The CST–Polα/primase complex is essential for telomere maintenance and functions to counteract resection at double-strand breaks. In addition to its telomeric function, CST–Polα/primase performs an analogous fill-in reaction at resected double-strand breaks (DSBs). We report a 4.6-Å resolution cryo-EM structure of human CST–Polα/primase, captured prior to catalysis in a recruitment state stabilized by chemical cross-linking. Our structure reveals an evolutionarily conserved interaction between the C-terminal domain of the catalytic POLA1 subunit and an N-terminal expansion in metazoan CTC1.

We purified Polα/primase lacking POLA1N (referred to hereafter as PPΔN), reconstituted a CST–PPΔN(–ssDNA) complex as for full-length Polα/primase (referred to hereafter as PPFL), and collected cryo-EM data. We used 131,850 particles to generate the final map with a global resolution of 4.6 Å. The ssDNA was included in the complex, as evidenced by the native gel of the GraFix fractions, but no reliable density could be found for it owing to the low resolution of CST in the cryo-EM map. After initial rigid-body docking followed by flexible fitting and refinement, the overall conformations of the two subcomplexes did not show major changes from their structures in isolation. Thus, we conclude that our structure likely captures a recruitment state of the complex that forms prior to active RNA and DNA synthesis by Polα/primase. The primary interaction interface observed in our structure occurs between the C-terminal domain of POLA1 (POLA1CTD, 1,265–1,462 aa) and the N-terminal OB folds of CTC1. The resolution is limiting for rigorous analysis of amino acid interactions, and analysis of surface electrostatic potential suggests that this interface is not driven by a dominant hydrophobic or charged interaction, but rather by shape complementarity of the two proteins, burying 1,250 Å2 of solvent-accessible surface area. The CRL and one Zn2+-binding domain in POLA1CTD form the module that fits into a complementary cleft in CTC1. CTC1OB-D, an elongated OB fold that shares no homology with known OB folds, forms the major interaction with POLA1CTD. V665 resides on a β-strand of CTC1OB-D, so it is plausible that a glycine substitution would destabilize the β-sheet and OB fold, disrupting the primary interaction.

> METFDPTELPELLKLYYRRLFPYSQYYRWLNYGGVIKNYFQHREFSFTLKDDIYIRYQSFNNQSDLEKEMQKMNPYKIDIGAVYSHRPNQHNTVKLGAFQAQEKELVFDIDMTDYDDVRRCCSSADICPKCWTLMTMAIRIIDRALKEDFGFKHRLWVYSGRRGVHCWVCDESVRKLSSAVRSGIVEYLSLVKGGQDVKKKVHLSEKIHPFIRKSINIIKKYFEEYALVNQDILENKESWDKILALVPETIHDELQQSFQKSHNSLQRWEHLKKVASRYQNNIKNDKYGPWLEWEIMLQYCFPRLDINVSKGINHLLKSPFSVHPKTGRISVPIDLQKVDQFDPFTVPTISFICRELDAISTNEEEKEENEAESDVKHRTRDYKKTSLAPYVKVFEHFLENLDKSRKGELLKKSDLQKDF;> GGSMEFSGRKWRKLRLAGDQRNASYPHCLQFYLQPPSENISLIEFENLAIDRVKLLKSVENLGVSYVKGTEQYQSKLESELRKLKFSYRENLEDEYEPRRRDHISHFILRLAYCQSEELRRWFIQQEMDLLRFRFSILPKDKIQDFLKDSQLQFEAISDEEKTLREQEIVASSPSLSGLKLGFESIYKIPFADALDLFRGRKVYLEDGFAYVPLKDIVAIILNEFRAKLSKALALTARSLPAVQSDERLQPLLNHLSHSYTGQDYSTQGNVGKISLDQIDLLSTKSFPPCMRQLHKALRENHHLRHGGRMQYGLFLKGIGLTLEQALQFWKQEFIKGKMDPDKFDKGYSYNIRHSFGKEGKRTDYTPFSCLKIILSNPPSQGDYHGCPFRHSDPELLKQKLQSYKISPGGISQILDLVKGTHYQVACQKYFEMIHNVDDCGFSLNHPNQFFCESQRILNGGKDIKKEPIQPETPQPKPSVQKTKDASSALASLNSSLEMDMEGLEDYFSEDS;> GPGSADEEQVFHFYWLDAYEDQYNQPGVVFLFGKVWIESAETHVSCCVMVKNIERTLYFLPREMKIDLNTGKETGTPISMKDVYEEFDEKIATKYKIMKFKSKPVEKNYAFEIPDVPEKSEYLEVKYSAEMPQLPQDLKGETFSHVFGTNTSSLELFLMNRKIKGPCWLEVKSPQLLNQPVSWCKVEAMALKPDLVNVIKDVSPPPLVVMAFSMKTMQNAKNHQNEIIAMAALVHHSFALDKAAPKPPFQSHFCVVSKPKDCIFPYAFKEVIEKKNVKVEVAATERTLLGFFLAKVHKIDPDIIVGHNIYGFELEVLLQRINVCKAPHWSKIGRLKRSNMPKLGGRSGFGERNATCGRMICDVEISAKELIRCKSYHLSELVQQILKTERVVIPMENIQNMYSESSQLLYLLEHTWKDAKFILQIMCELNVLPLALQITNIAGNIMSRTLMGGRSERNEFLLLHAFYENNYIVPDKQIFRKPQQKLGDEDEEIDGDTNKYKKGRKKAAYAGGLVLDPKVGFYDKFILLLDFNSLYPSIIQEFNICFTTVQRVASEAQKVTEDGEQEQIPELPDPSLEMGILPREIRKLVERRKQVKQLMKQQDLNPDLILQYDIRQKALKLTANSMYGCLGFSYSRFYAKPLAALVTYKGREILMHTKEMVQKMNLEVIYGDTDSIMINTNSTNLEEVFKLGNKVKSEVNKLYKLLEIDIDGVFKSLLLLKKKKYAALVVEPTSDGNYVTKQELKGLDIVRRDWCDLAKDTGNFVIGQILSDQSRDTIVENIQKRLIEIGENVLNGSVPVSQFEINKALTKDPQDYPDKKSLPHVHVALWINSQGGRKVKAGDTVSYVICQDGSNLTASQRAYAPEQLQKQDNLTIDTQYYLAQQIHPVVARICEPIDGIDAVLIATWLGLDPTQFRVHHYHKDEENDALLGGPAQLTDEEKYRDCERFKCPCPTCGTENIYDNVFDGSGTDMEPSLYRCSNIDCKASPLTFTVQLSNKLIMDIRRFIKKYYDGWLICEEPTCRNRTRHLPLQFSRTGPLCPACMKATLQPEYSDKSLYTQLCFYRYIFDAECALEKLTTDHEKDKLKKQFFTPKVLQDYRKLKNTAEQFLSRSGYSEVNLSKLFAGCAVKS;> MSASAQQLAEELQIFGLDCEEALIEKLVELCVQYGQNEEGMVGELIAFCTSTHKVGLTSEILNSFEHEFLSKRLSKARHSTCKDSGHAGARDIVSIQELIEVEEEEEILLNSYTTPSKGSQKRAISTPETPLTKRSVSTRSPHQLLSPSSFSPSATPSQKYNSRSNRGEVVTSFGLAQGVSWSGRGGAGNISLKVLGCPEALTGSYKSMFQKLPDIREVLTCKIEELGSELKEHYKIEAFTPLLAPAQEPVTLLGQIGCDSNGKLNNKSVILEGDREHSSGAQIPVDLSELKEYSLFPGQVVIMEGINTTGRKLVATKLYEGVPLPFYQPTEEDADFEQSMVLVACGPYTTSDSITYDPLLDLIAVINHDRPDVCILFGPFLDAKHEQVENCLLTSPFEDIFKQCLRTIIEGTRSSGSHLVFVPSLRDVHHEPVYPQPPFSYSDLSREDKKQVQFVSEPCSLSINGVIFGLTSTDLLFHLGAEEISSSSGTSDRFSRILKHILTQRSYYPLYPPQEDMAIDYESFYVYAQLPVTPDVLIIPSELRYFVKDVLGCVCVNPGRLTKGQVGGTFARLYLRRPAADGAERQSPCIAVQVVRI;> GPGSMAAGRAQVPSSEQAWLEDAQVFIQKTLCPAVKEPNVQLTPLVIDCVKTVWLSQGRNQGSTLPLSYSFVSVQDLKTHQRLPCCSHLSWSSSAYQAWAQEAGPNGNPLPREQLLLLGTLTDLSADLEQECRNGSLYVRDNTGVLSCELIDLDLSWLGHLFLFPRWSYLPPARWNSSGEGHLELWDAPVPVFPLTISPGPVTPIPVLYPESASCLLRLRNKLRGVQRNLAGSLVRLSALVKSKQKAYFILSLGRSHPAVTHVSIIVQVPAQLVWHRALRPGTAYVLTELRVSKIRGQRQHVWMTSQSSRLLLLKPECVQELELELEGPLLEADPKPLPMPSNSEDKKDPESLVRYSRLLSYSGAVTGVLNEPAGLYELDGQLGLCLAYQQFRGLRRVMRPGVCLQLQDVHLLQSVGGGTRRPVLAPCLRGAVLLQSFSRQKPGAHSSRQAYGASLYEQLVWERQLGLPLYLWATKALEELACKLCPHVLRHHQFLQHSSPGSPSLGLQLLAPTLDLLAPPGSPVRNAHNEILEEPHHCPLQKYTRLQTPSSFPTLATLKEEGQRKAWASFDPKALLPLPEASYLPSCQLNRRLAWSWLCLLPSAFCPAQVLLGVLVASSHKGCLQLRDQSGSLPCLLLAKHSQPLSDPRLIGCLVRAERFQLIVERDVRSSFPSWKELSMPGFIQKQQARVYVQFFLADALILPVPRPCLHSATPSTPQTDPTGPEGPHLGQSRLFLLCHKEALMKRNFCVPPGASPEVPKPALSFYVLGSWLGGTQRKEGTGWGLPEPQGNDDNDQKVHLIFFGSSVRWFEFLHPGQVYRLIAPGPATPMLFEKDGSSCISRRPLELAGCASCLTVQDNWTLELESSQDIQDVLDANKSLPESSLTDLLSDNFTDSLVSFSAEILSRTLCEPLVASLWMKLGNTGAMRRCVKLTVALETAECEFPPHLDVYIEDPHLPPSLGLLPGARVHFSQLEKRVSRSHNVYCCFRSSTYVQVLSFPPETTISIPLPHIYLAELLQGGQSPFQATASCHIVSVFSLQLFWVCAYCTSICRQGKCTRLGSTCPTQTAISQAIIRLLVEDGTAEAVVTCRNHHVAAALGLCPREWASLLDFVQVPGRVVLQFAGPGAQLESSARVDEPMTMFLWTLCTSPSVLRPIVLSFELERKPSKIVPLEPPRLQRFQCGELPFLTHVNPRLRLSCLSIRESEYSSSLGILASSC;> MQPGSSRCEEETPSLLWGLDPVFLAFAKLYIRDILDMKESRQVPGVFLYNGHPIKQVDVLGTVIGVRERDAFYSYGVDDSTGVINCICWKKLNTESVSAAPSAARELSLTSQLKKLQETIEQKTKIEIGDTIRVRGSIRTYREEREIHATTYYKVDDPVWNIQIARMLELPTIYRKVYDQPFHSSALEKEEALSNPGALDLPSLTSLLSEKAKEFLMENRVQSFYQQELEMVESLLSLANQPVIHSASSDQVNFKKDTTSKAIHSIFKNAIQLLQEKGLVFQKDDGFDNLYYVTREDKDLHRKIHRIIQQDCQKPNHMEKGCHFLHILACARLSIRPGLSEAVLQQVLELLEDQSDIVSTMEHYYTAF;> MMLPKPGTYYLPWEVSAGQVPDGSTLRTFGRLCLYDMIQSRVTLMAQHGSDQHQVLVCTKLVEPFHAQVGSLYIVLGELQHQQDRGSVVKARVLTCVEGMNLPLLEQAIREQRLYKQERGGSQ> SNAMYKYITILGAAGQIAQKLTATLLTYTDMHITLYGRQLKTRIPPEIIDHERVTVIEGSFQNPGKLEQAVTNAEVVFVGAMESGS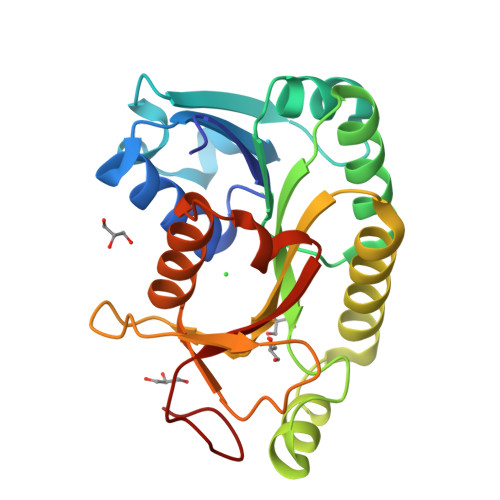DMASIVKALSRKNIRRVIGVSMAGLSGEFPVALEKWTFDNLPISYVQGERQARNVLRESNLNYTILRLTWLYNDPEKTDYELIPEGAQFNDAQVSREAVVKAIFDILHAADETPFHRTSIGVGEPGTHYDKPSFH>RYRVEYHLKSHRKDEFIDWVKGLLASPFVLHAVSHEGDYNDDLATTQRVRSQYADIFKDIEGLIKDKIEFDSRNMSQDEIEDGASSQSLNILGQSRLNLLVPSIGTFFTELPLEQAFLWEDSQRAISARRMVAPSFNDIRHILNTAQIFHFKKQENLHNGKVLRLVTFDGDVTLYEDGGSLVYTNPVIPYILKLLRCGINVGIVTAAGYDEAGTYENRLKGLIVALHDSTDIPVSQKQNLTIMGGESSYLFRYYEDPEEDNFGFRQIDKEEWLLPRMKAWSLEDVEKTLDFAERTLNRLRKRLNLPSEISIIRKVRAVGIVPGERYDEASKRQVPVKLDREQLEEIVLTLQNTLESFAPSRRIQFSCFDGGSDVWCDIGG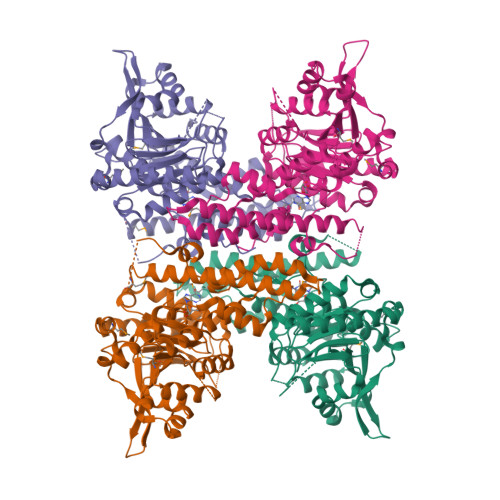KDLGVRSLQQFYNPESPIQPSETLHVGDQFAPVGSANDFKARLAGCTLWIASPQETVNYLHRLLETDHHHHHHHH[4x]>MRESAAQKFQRQHMDPDGSSINSPTYCNQMMKRRDMTNGSCKPVNTFVHEPLADVQAVCSQENVTCKNRKSNCYKSSSALHITDCHLKGNSKYPNCDYKTTQYQKHIIVACEGNPYVPVHFDATV[4x]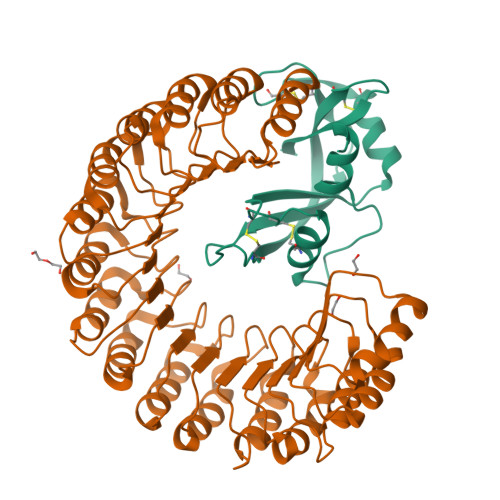;>MMSLDIQCEQLSDARWTELLPLIQQYEVVRLDDCGLTEVRCKDISSAVQANPALTELSLRTNELGDGGVGLVLQGLQNPTCKIQKLSLQNCGLTEAGCGILPGMLRSLSTLRELHLNDNPMGDAGLKLLCEGLQDPQCRLEKLQLEYCNLTATSCEPLASVLRVKADFKELVLSNNDLHEPGVRILCQGLKDSACQLESLKLENCGITAANCKDLCDVVASKASLQELDLSSNKLGNAGIAALCPGLLLPSCKLRTLWLWECDITAEGCKDLCRVLRAKQSLKELSLASNELKDEGARLLCESLLEPGCQLESLWIKTCSLTAASCPYFCSVLTKSRSLLELQMSSNPLGDEGVQELCKALSQPDTVLRELWLGDCDVTNSGCSSLANVLLANRSLRELDLSNNCMGGPGVLQLLESLKQPSCTLQQLVLYDIYWTNEVEEQLRALEEERPSLRIIS[4x]>GSPGLDGICQSTSNHLWLLSDILGQGATANVFRGRHKKTGDLYAVKVFNNISFLRPVDVQMREFEVLKKLNHKNIVKLFAIEEETTTRHKVLIMEFCPCGSLYTVLEEPSNAYGLPESEFLIVLRDVVGGMNHLRENGIVHRDIKPGNIMRVIGEDGQSVYKLTDFGAARELEDDEQFVALYGTEEYLHPDMYERAVLRKDHQKKYGATVDLWSVGVTFYHAATGSLPFRPFEGPRRNKEVMYKIITGKPSGAISGVQKAENGPIDWSGDMPLSCSLSQGLQALLTPVLANILEADQEKCWGFDQFFAETSDVLHRMVIHVFSLQHMTAHKIYIHSYNTAAVFHELVYKQTKIVSSNQELIYEGRRLVLELGRLAQHFPKTTEENPIFVTSREQLNTVGLRYEKISLPKIHPRYDLDGDASMAKAV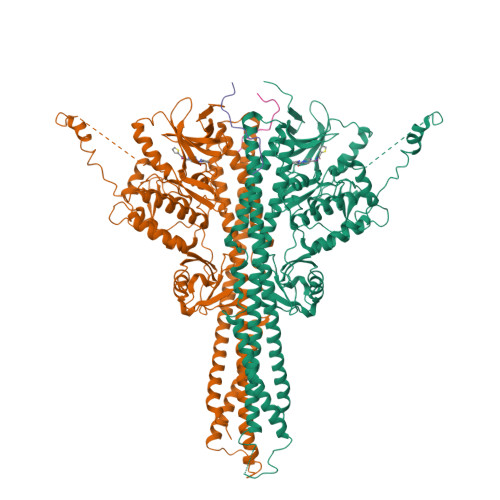TGVVCYACRTASTLLLYQELMRKGVRWLVELVKDDYNETVHKKTEVVITLDFCIRNIEKTVKVYEKLMKVNLEAAELGEISDIHTKLLRLSSSQGTIESSLQDISSRLSPGGLLADTWAHQEGTHPRDRNVEKLQVLLNCITEIYYQFKKDKAERRLAYNEEQIHKFDKQKLYYHATKAMSHFSEECVRKYEAFKDKSEEWMRKMLHLRKQLLSLTNQCFDIEEEVSKYQDYTNELQET[2x];>[2x]STWGSLKTSAVPSTSTMSQEPELLISGMEKPLPLRTDFS>[2x]AETAKPATDATKAANDALLKELPFDDKTSFDLAHKGFIAPLPAEPIKGEKGNMIWDPSKYGFIKEGEAAPDTTNPSLWRQSQLINISGLFEVTDGIYQVRNYDLSNMTIVEGKDGITIFDPLISQETAKAALDLYYKHRPKKPVVAVIYTHSHVDHYGGVRGVVDEADVKAGKVKIYAPLGFLEHAVAENVMAGTAMSRRASYMYGNLLPPDAKGQLGAGLGTT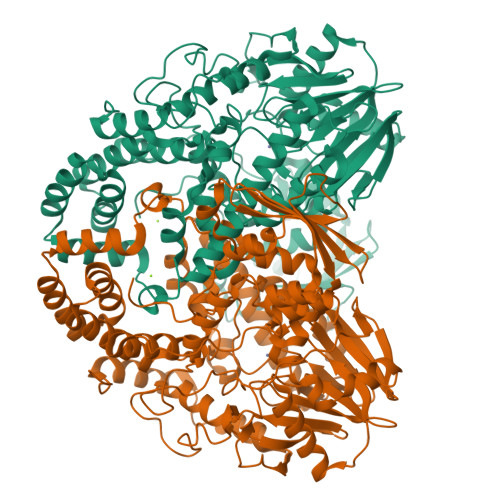TSAGTVTLIPPTDIIKETGETHVIDGLTYEFMYAPGSEAPAEMLYYIKEKKALNAAEDSTHTLHNTYSLRGAKIRDPLAWSKYLNEALKLWGDDVQVMYAMHHWPVWGNKEVREQLSLQRDMYRYINDETLRLANKGYTMTEIAEQVKLPKKIATKFSNRGYYGSLNHNVKATYVLYLGWFIGNPATLWELPPADKAKRYVEMMGGADAVLKKAKEYYDKGDFRWVAEVVNHVVFAEPNNQAAKNMQADALEQLGYQAESGPWRNFYLTGAQELRNGVQQLPTPDTASPDTVKAMDLDLFFDFLAMRLKGPDVADKHITLNLDFTDLKQKYTLEMVNGVLNHTEGMQAKNADATVTLTRETLNNVMLKQTTLKDAESSGDIKIEGDKGKLEELMSYMDNFDFWFNIVTP> ETFEEFTARYEKEFDEAYDLFEVQRVLNNCFSYDLVPAPAVIEKALRAARRVNDLPTAIRVFEALKYKVENEDQYKA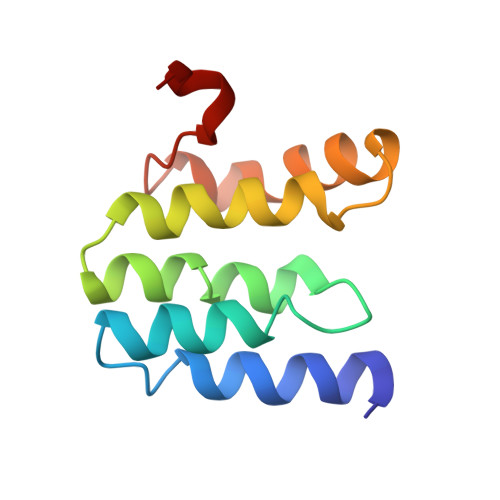YLDELKDVRQELGVPLKEELFP> ARDCPLV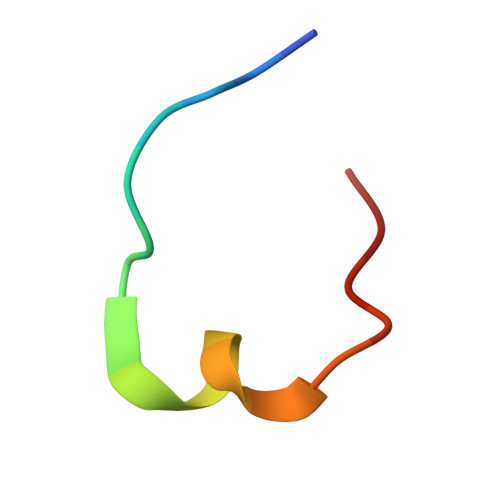NPLCLHPGWTC> SRDTKWLTLEVCREFQRGTCSRPDTECKFAHPSKSCQVENGRVIACFDSLKGRCSRENCKYLHPP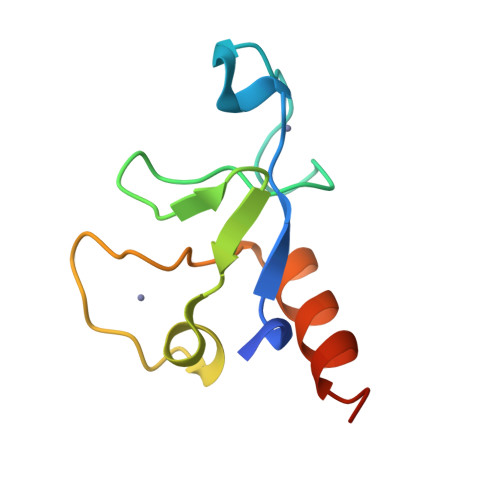PHLKTQLEINGRNNLIQQ> MSISILKDK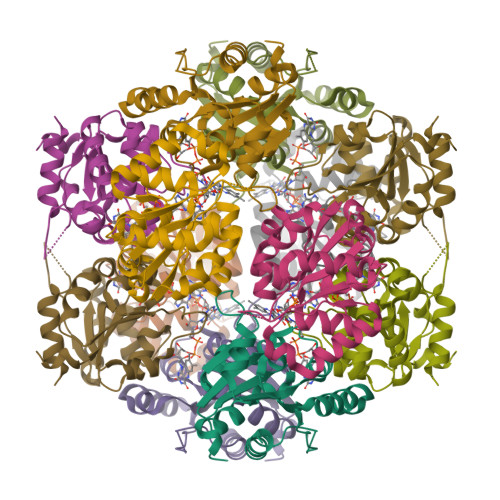KLLIGICGSISSVGISSYLLYFKSFFKEIRVVMTKTAEDLIPAHTVSYFCDHVYSEHGENGKRHSHVEIGRWADIYCIIPATANILGQTANGVAMNLVATTVLAHPHNTIFFPNMNDLMWNKTVVSRNIEQLRKDGHIVIEPVEIMAFEIATGTRKPNRGLITPDKALLAIEKGFKERTKHPSLT> SNADDMIILKGVNIFPIQIETILLQFKELGSDYLITLETAESNDEMTVEVELSQLFTDDYGRLQALTREITRQ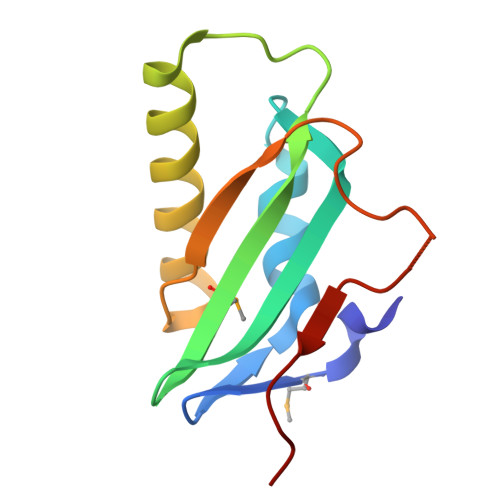LKDEILVTPRVKLVPKGALPKSEGKAVRVKDLRKTF>MTTQAPTFTQPLQSVVVLEGSTATFEAHISGFPVPEVSWFRDGQVISTSTLPGVQISFSDGRAKLTIPAVTKANSGRYSLKATNGSGQATSTAELLVKAETAPPNFVQRLQSMTVRQGSQVRLQVRVTGIPTPVVKFYRDGAEIQSSLDFQISQEGDLYSLLIAEAYPEDSGTYSVNATNSVGRATSTAELLVQ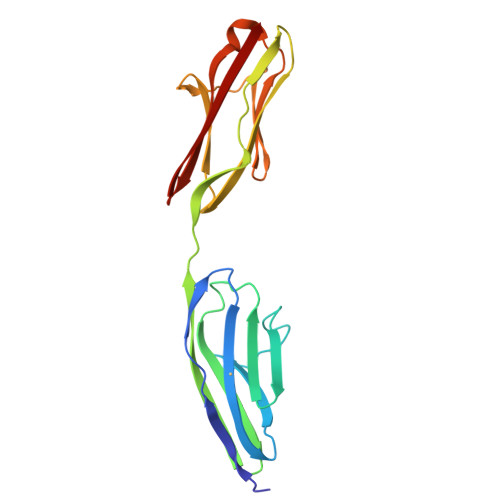[3x]Bacterial RNA polymerase (RNAP) holoenzyme initiates transcription by recognizing the conserved –35 and –10 promoter elements that are optimally separated by a 17-bp spacer. The MerR family of transcriptional regulators activate suboptimal 19–20 bp spacer promoters in response to myriad cellular signals, ranging from heavy metals to drug-like compounds. Here we report one crystal structure of a multidrug-sensing MerR family regulator EcmrR and nine cryo-electron microscopy structures that capture the EcmrR-dependent transcription process from promoter opening to initial transcription to RNA elongation. These structures reveal that EcmrR is a dual ligand-binding factor that reshapes the suboptimal 19-bp spacer DNA to enable optimal promoter recognition, sustains promoter remodeling to stabilize initial transcribing complexes, and finally dissociates from the promoter to reverse DNA remodeling and facilitate the transition to elongation.

Although the CTDs of EcmrR (residues 112–269) and BmrR are highly divergent in sequence, their three-dimensional structures are readily superimposable. Both CTDs belong to GyrI-like domain family, a well-characterized motif that is adapted for multidrug binding. Dual site-binding is also observed in the 1.4 Å EcmrR CTD crystal structure, wherein both sites are occupied by cetyltrimethylammonium cation (CTA+), a cationic detergent in the crystallization solution. The overall shape and pocket residue conformations of site I remain largely unchanged between the CTA+- and TPSb+-bound forms except for a slight retraction of the E185 side chain to avoid clashes with one of the phenyl rings in TPSb+. In comparison, site II is relatively flexible and undergoes significant conformational changes between its un-liganded, CTA+-bound and CHAPSO-bound forms. Y174 and R220, which partially occupy site II in the absence of ligand, gradually lift up as a ligand binds and as the bound ligand gets bulkier. The two ligand-binding sites in EcmrR are approximately symmetric about a pseudo-two-fold axis of the triangle-shaped EcmrR CTD. A glutamate residue in each site (E185 and E243) dictates the preference for cationic compounds, while the lack of a positive charge in the tetracyclic sterol head of CHAPSO is compensated for by hydrogen bonds between its hydroxyl groups and polar residues on the surface of site II and extensive hydrophobic interactions in the ligand-binding pocket.

>[4x]SMLYQAALKEIPECIVYSKRFIVPDFSSYIKLIPPIGQEVMKANPGLTLTTPAYCFTLYHDKEYKEKNMDVEFCEAVNDFGKNEGNIIFQVIPAITAVTVIHKGPYDSLRNAYIYLMQWVEDNGYLLTNSPRESYIDGIWNKQDSAEWMTEIQFPVEKV> MTDNNKSSKTPNAWIAIDHNFSRAQVLTYYTLQLKGEHSLHQAISDNDWILVLDTTGNITRVGRILRIRSDLETTTIFFDRMLQVKSVVSIGITPFKFPPNDRAGRIQWTDFIETLPKELHITIADIPKIEDQTYIRELLQLAVMDDLLGPAGGPNELIVDMGVRDRYLVGKLAPREAAERGQEFPIDAEDIEDEEPDLIVKAKTAKVNSPSVLGSGETDTAEEIDAASNQSLVPSSLGMTFCVDGDVDRVEIEARWGRYERVPNDEHQFFKSNGQKAKVWKRIPCGGKIVLPLIEGSISHNAPDSTSPEVRVQGSIRAKNDNGDRLITLFLVNAQEEPDTNRDTAWVFQPELIVRAAKDAAKPAIFRRRPVLDADGMDPEREALEMIYRDRVEFAVGHGVAVHAEIADDVTLATEVRTTVMPQYEVQATETPGLELSDRPAMREMVSSGLLDMQRLATLDIDPLVDALSVLTNDYATWIDEQNLNVSSKAKGFDTQAQTAINRCQEIHTRLQEGINTLKSNENALAAFRFANQAMATQRIRSLYALAMRRGEDVTLDKFDVLKNRSWRPFQLAFLLLSIPSLADPCHPDRVKPIEAYADLLWFPTGGGKTEAYLGVAAFTMAIRRMQGNLGGYDSSRGLTVIMRYTLRLLTLQQFQRATALICAMEVLRREALNKGDKSLGTEPFTIGLWVGNKVTPGTTEDSHNAIEKTRNPGSYNAGTASPVQLTSCPWCGTEIVPGQDVEVKKDKAGGRTFVYCGDKKGRCEFSKGKSSTQPHPGIPVLVVDEEIYHRPPTMMIATVDKFAMMAWRGQVRTLFGRVEKECERHGLLWPGANCTGNHQAFKGQPSAKVKAIPPIRPPDLIIQDEFHLISGPLGTMVGLYETAVDELCSWTLNGKTVKPKIIASTATVRKAKEQVNNVFMRQVSVFPPHGLDVEDNFFSVQRHIKDKFGRRYLGVCSPGSSRPAMLIRVYTAFLTAAQELFDHFGEPADPYMTMVGYFNSLRELGGMKRLAEDDVQTRSYRVQMSMVERPALAQRSVNNIRELTSRVSSQDIPKYLDNLEVKFKAEFDSSAGKYVTKWQEGDTRAIDVVLATNMLSVGVDVNRLGLMAVNGQPKGTAEYIQATSRVGRSFPGLVCTVLTWARPRDLSHYETFEHYHATFYKHVEAQSVTPFSPRAMDRGLTGSLLSLMRLKNNEFSPNEGAGKLDMSNQSELAHAIEVLATRAGNVAEDNARKLLAENELKERADEWAKEASKGGRILGYEKRGPDKDKTVALIKSPGLQAWDNWTVPMSMREVESGVRLIMDTKFIKDDHDWKPRPATKDE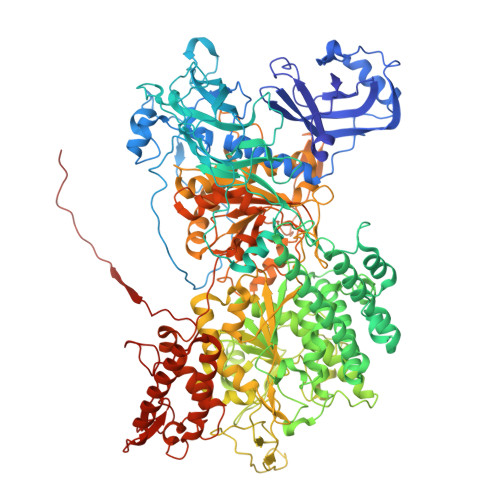D>[2x]LSKVVIRRLPPTLTKEQLQEHLQPMPEHDYFEFFSNDTSLYPHMYARAYINFKNQEDIILFRDRFDGYVFLDNKGQEYPAIVEFAPFQKAA;>[2x]RPPLQEYVRKLLYKDLSKVTTEKVLRQMRKLPWQDQEVKDYVICCM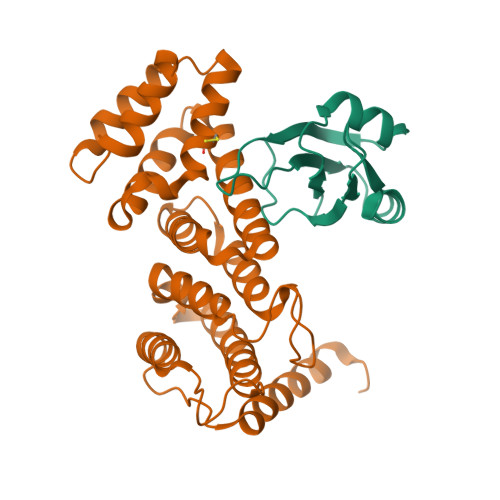INIWNVKYNSIHCVANLLAGLVLYQEDVGIHVVDGVLEDIRLGMEVNQPKFNQRRISSAKFLGELYNYRMVESAVIFRTLYSFTSFGVNPDGSPSSLDPPEHLFRIRLVCTILDTCGQYFDRGSSKRKLDCFLVYFQRYVWWKKSLEVWTKDHPFPIDIDYMISDTLELLRPKIKLCNSLEESIRQVQDLEREFLIKLGLVN2-azanyl-3-(2,6-dimethyl-3-oxidanyl-phenyl)-5-pyridin-4-yl-benzamide | 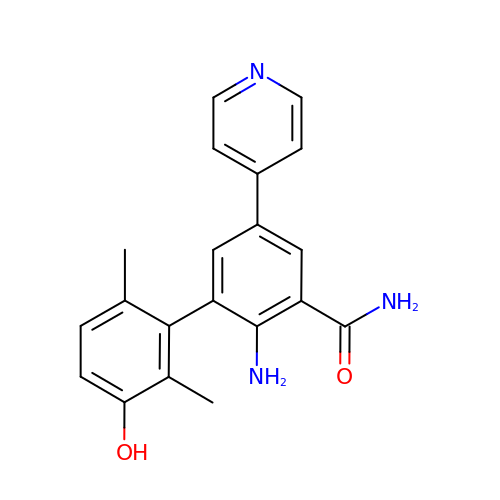C20 H19 N3 O2 | WMCIJTOVEOXHKF-UHFFFAOYSA-N>[2x]MQNITINTPRKRIYHNILETIGGTPLVELHGVTDHPSIKKNTKILVKLECFNPMSSVKDRVGFNIIYQAIKDGRLKPGMEIIEATSGNTGIGLCQAGAVFGYPVNIVMPSTMSVERQMIMKAFGANLVLSDGTKGMPGAIAKYEELIKQHPNKYFPANQFGNPDNTAAHVYTANEIWEDTNGEVDIIVSAVGTAGTVIGVGEN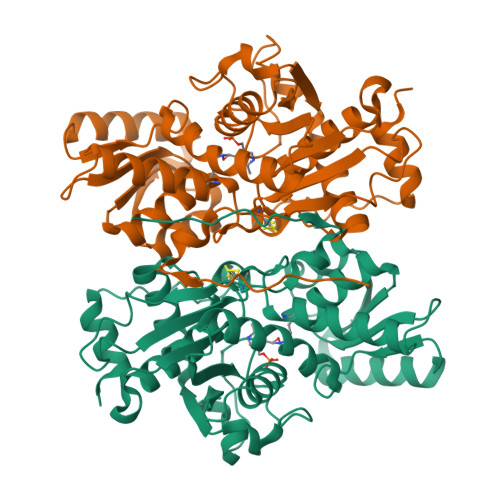LKKKKKGVKVVAVEPAESAVLSGKPKGPHGIQGIGAGFVTDIYKKEVVDEITPIKTQDAWKMARAVVKYDGIMCGMSSGAAILAGLKEAGKVENEGKTIVIILPDCGERYLSTDLYKTIEEGTKQQVLDSLLLHH>NARKVQMGAKDATPVPCGRWAKILEKDKRTQQMRMQRLKAKLQMPFQSGEFKALTRRLQVEPRLLSKQMAGCLEDCTRQAPESPWEEQLARLLQEAPGKLSLDVEQAPSGQHSQAQLSGQQQRLLAFFKCCLLTDQLPLAHHLLVVHHGQRQKRKLLTLDMYNAVMLGWARQGAFKELVYVLFMVKDAGLTPDLLSYAAALQCMGRQDQDAGTIERCLEQMSQEGLKLQALFTAVLLSEEDRATVLKAVHKVKPTFSLPPQLPPPVNTSKLLRDVYAKDGRVSYPKLHLPLKTLQCLFEKQLHMELASRVCVVSVEKPTLPSKEVKHARKTLKTLRDQWEKALCRALRETKNRLEREVYEGRFSLYPFLCLLDEREVVRMLLQVLQALPAQGESFTTLARELSARTFSRHVVQRQRVSGQVQALQNHYRKYLCLLASDAEVPEPCLPRQYWEALGAPEALREQPWPLPVQMELGKLLAEMLVQATQMPCSLDKPHRSSRLVPVLYHVYSFRNVQQIGILKPHPAYVQLLEKAAEPTLTFEAVDVPMLCPPLPWTSPHSGAFLLSPTKLMRTVEGATQHQELLETCPPTALHGALDALTQLGNCAWRVNGRVLDLVLQLFQAKGCPQLGVPAPPSEAPQPPEAHLPHSAAPARKAELRRELAHCQKVAREMHSLRAEALYRLSLAQHLRDRVFWLPHNMDFRGRTYPCPPHFNHLGSDVARALLEFAQGRPLGPHGLDWLKIHLVNLTGLKKREPLRKRLAFAEEVMDDILDSADQPLTGRKWWMGAEEPWQTLACCMEVANAVRASDPAAYVSHLPVHQDGSCNGLQHYAALGRDSVGAASVNLEPSDVPQDVYSGVAAQVEVFRRQDAQRGMRVAQVLEGFITRKVVKQTVMTVVYGVTRYGGRLQIEKRLRELSDFPQEFVWEASHYLVRQVFKSLQEMFSGTRAIQHWLTESARLISHMGSVVEWVTPLGVPVIQPYRLDSKVKQIGGGIQSITYTHNGDISRKPNTRKQKNGFPPNFIHSLDSSHMMLTALHCYRKGLTFVSVHDCYWTHAADVSVMNQVCREQFVRLHSEPILQDLSRFLVKRFCSEPQKILEASQLKETLQAVPKPGAFDLEQVKRSTYFFS[2x];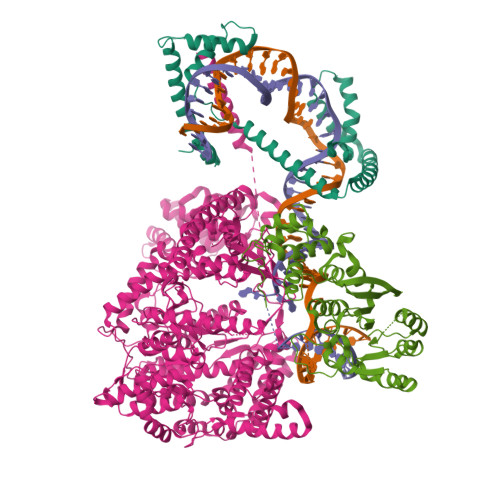>NASSVLASSPKKPVSSYLRFSKEQLPIFKAQNPDAKTTELIRRIAQRWRELPDSKKKIYQDAYRAEWQVYKEEISRFKEQLTPSQIMSLEKEIMDKHLKRKAMTKKKELTLLGKPKRPRSAYNVYVAERFQEAKGDSPQEKLKTVKENWKNLSDSEKELYIQHAKEDETRYHNEMKSWEEQMIEVGRKDLLRRTIKKQRKYGAEE[2x];>NARFCILGSEAATRKHLPARNHCGLSDSSPQLWPEPDFRNPPRKASKASLDFKRYVTDRRLAETLAQIYLGKPSRPPHLLLECNPGPGILTQALLEAGAKVVALESDKTFIPHLESLGKNLDGKLRVIHCDFFKLDPRSGGVIKPPAMSSRGLFKNLGIEAVPWTADIPLKVVGMFPSRGEKRALWKLAYDLYSCTSIYKFGRIEVNMFIGEKEFQKLMADPGNPDLYHVLSVIWQLACEIKVLHMEPWSSFDIYTRKGPLENPKRRELLDQLQQKLYLIQMIPRQNLFTKNLTPMNYNIFFHLLKHCFGRRSATVIDHLRSLTPLDARDILMQIGKQEDEKVVNMHPQDFKTLFETIERSKDCAYKWLYDETLEDR[2x]>[6x]MISNEEQTPLLKKINPTE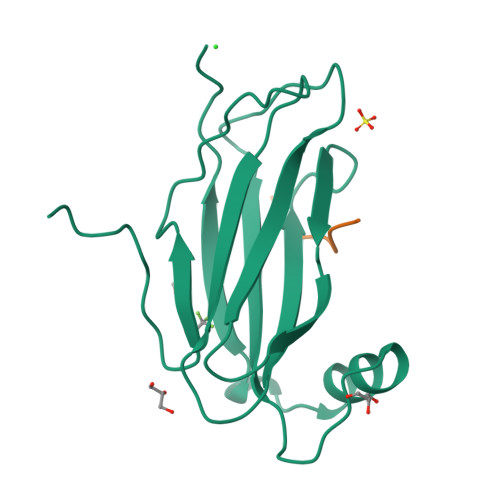STSKAEENEKVDSKVKAFKKPLSVFKGPLLHISPAEELYFGSTESGEKKTLIVLTNVTKNIVAFKVRTTAPEKYRVKPSNSSCDPGASVDIVVSPHGGLTVSAQDRFLIMAAEMEQSSGTGPAELTQFWKEVPRNKVMEHRLRCHTVESSKPNTLTLKDNAFNMSDKTSEDICLQLSRLLESNRKLEDQVQRHHHHHH;>[5x]GAMRSILSEDEFYDALSDSES>[2x]MHHHHHHHHHHGENLYFQGSDNIISFDHVTFTYPDSPRPALSDLSFAIERGSWTALIGHNGSGKSTVSKLINGLLAPDDLDKSSITVDGVKLGADTVWEVREKVGIVFQNPDNQFVGATVSDDVAFGLENRAVPRPEMLKIVAQAVADVGMADYADSEPSNLSGGQKQRVAIAGILAVKPQVIILDESTSMLDPEGKEQILDLVRKIKEDNNLTVISITHDLEEAAGADQVLVLDDGQLLDQGKPEEIFPKVEMLKRIGLDIPFVYRLKQLLKERGIVLPDEIDDDEKLVQSLWQLNS;>[2x]MAIKFENVSYVYSPGSPLEAIGLDQLNFSLEEGKFIALVGHTGSGKSTLMQHFNALLKPTSGKIEIAGYTITPETGNKGLKDLRRKVSLAFQFSEAQLFENTVLKDVEYGPRNFGFSEDEAREAALKWL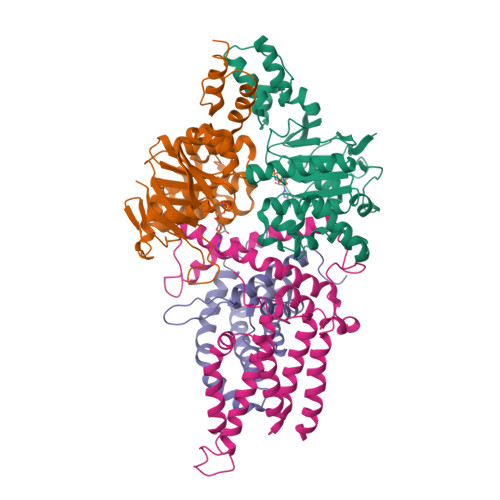KKVGLKDDLIEHSPFDLSGGQMRRVALAGVLAYEPEIICLDEPAAGLDPMGRLEMMQLFKDYQAAGHTVILVTHNMDDVADYADDVLALEHGRLIKHASPKEVFKDSEWLQKHHLAEPRSARFAAKLEAAGLKLPGQPLTMPELADAIKQSLKGGEHE;>MKSESKVSSKLELRELVLLAMVIAIKVILGQFKVGNATLQVGLGFIGSVMLGYLFGPWWGFAGGALSDLVSSVIFGNLGGFFIGFTLTAALGPMIYGFFLYKQPIQIWRVIASVICVTVICNIGLNTLWVSMMYGINFMVALSSRILKEMITPWIQMVAVWFILEGLSRVKLSRKFWSHPQFEK[2x];>[2x]MSKIIIGRYLPGTTFVYRVDPRAKLLTTFYFIIMIFLANNWVSYLVISIFGLAYVFATGLKARVFWDGVKPMIWMIVFTSLLQTFFMAGGKVYWHWWIFTLSSEGLINGLYVFIRFAMIILVSTVMTVTTKPLEIADAMEWMLTPLKLFKVNVGMISLVISIALRFVPTLFDQTVKIMNAQRSRGADFNDGGLVKRAKSVVPMLVPLFIDSLEVALDLSTAMESRGYKGSEGRTRYRILEWSKVDLIPVAYCLLLTILMITTRKH> GPGSEFGTREFLTFEVPLNDSGSAGLGVSVKGNRSKENHADLGIFVKSII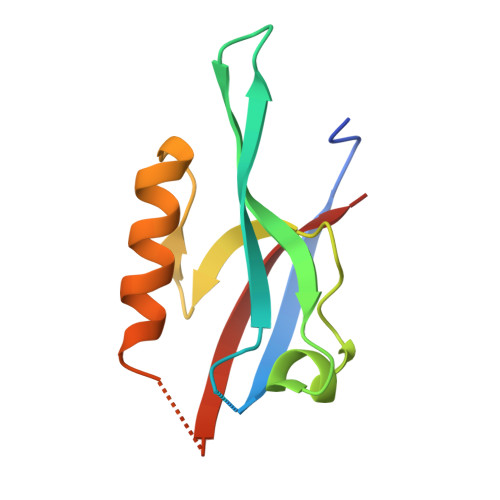NGGAASKDGRLRVNDQLIAVNGESLLGKANQEAMETLRRSMSTEGNKRGMIQLIVARRIS> MHHHHHHAAGIPMNNPAIKRIGNHITKSPEDKREYRGLELANGIKVLLISDPTTDKSSAALDVHIGSLSDPPNIAGLSHFCQHMLFLGTKKYPKENEYSQFLSEHAGSSNAFTSGEHTNYYFDVSHEHLEGALDRFAQFFLCPLFDESCKDREVNAVDSEHEKNVMNDAWRLFQLEKATGNPKHPFSKFGTGNKYTLETRPNQEGIDVRQELLKFHSAYYSSNLMAVCVLGRESLDDLTNLVVKLFSEVENKNVPLPEFPEHPFQEEHLKQLYKIVPI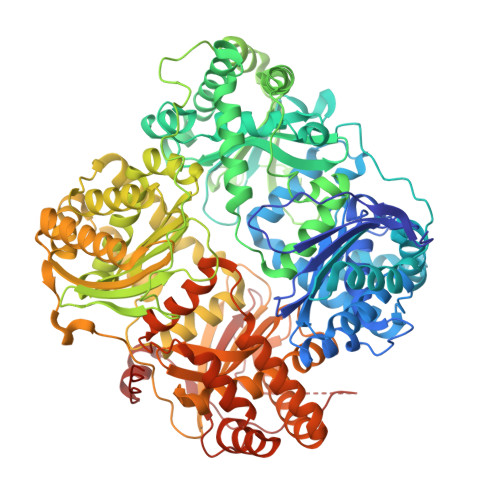KDIRNLYVTFPIPDLQKYYKSNPGHYLGHLIGHEGPGSLLSELKSKGWVNTLVGGQKEGARGFMFFIINVDLTEEGLLHVEDIILHMFQYIQKLRAEGPQEWVFQECKDLNAVAFRFKDKERPRGYTSKIAGILHYYPLEEVLTAEYLLEEFRPDLIEMVLDKLRPENVRVAIVSKSFEGKTDRTEEWYGTQYKQEAIPDEVIKKWQNADLNGKFKLPTKNEFIPTNFEILPLEKEATPYPALIKDTAMSKLWFKQDDKFFLPKACLNFEFFSPFAYVDPLHCNMAYLYLELLKDSLNEYAYAAELAGLSYDLQNTIYGMYLSVKGYNDKQPILLKKIIEKMATFEIDEKRFEIIKEAYMRSLNNFRAEQPHQHAMYYLRLLMTEVAWTKDELKEALDDVTLPRLKAFIPQLLSRLHIEALLHGNITKQAALGIMQMVEDTLIEHAHTKPLLPSQLVRYREVQLPDRGWFVYQQRNEVHNNCGIEIYYQTDMQSTSENMFLELFCQIISEPCFNTLRTKEQLGYIVFSGPRRANGIQGLRFIIQSEKPPHYLESRVEAFLITMEKSIEDMTEEAFQKHIQALAIRRLDKPKKLSAECAKYWGEIISQQYNFDRDNTEVAYLKTLTKEDIIKFYKEMLAVDAPRRHKVSVHVLAREMDSCPVVGEFPCQNDINLSQAPALPQPEVIQNMTEFKRGLPLFPLVKPHINFMAAKL> XKLRPVAM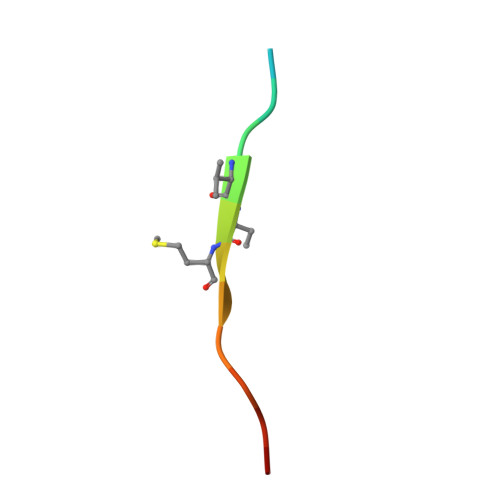VRPTVR>[6x]GCSSNYVMHTNDGRTIV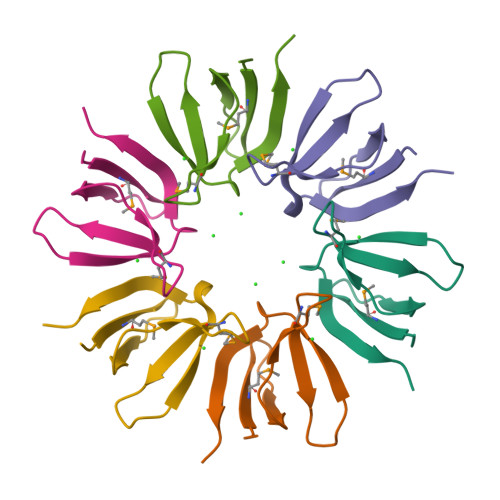TDGKPQTDNDTGMISYKDAWGNKQQINRSDVKQLGELDE> MGKRHRNLIDQITTWENLLDAYRKTSHGKRRTWGYLEFKEYDLANLLALQAELKAGNYERGPYREFLVYEPKPRLISALEFKDRLVQHALCNIVAPIFEAGLLPYTYACRPDKGTHAGVCHVQAELRRTRATHFLKSDFSKFFPSIDRAALYAMIDKKIHCAATRRLLRVVLPDEGVGIPIGSLTSQLFANVYGGAVDRLLHDELKQRHWARYMDDIVVLGDDPEELRAVFYRLRDFASERLGLKISHWQVAPVSRGINFLGYRIWPTHKLLRKSSVKRAKRKVANFIKHGEDESLQRFLASWSGHAQWADTHNLFTWMEEQYGIACH;>[5x]MEPIEEATKCYDQMLIVERYERVISYLYPIAQSIPRKHGVAREMFLKCLLGQVELFIVAGKSNQVSKL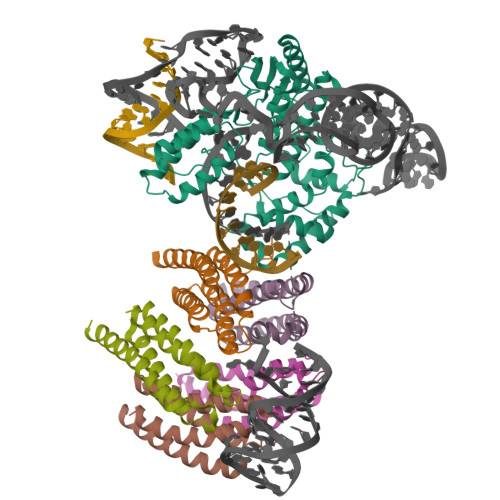YAADAGLAMLRFWLRFLAGIQKPHAMTPHQVETAQVLIAEVGRILGSWIARVNRKGTKVQVGEALVGDGNEVAHIDLIIGPRGSPAETAFCNGLVNNKHGFTSLLAVIAPNLPCKPNTLMFNKVTINDARQAVQMFGPAQHGVAMAVQDAVAEGIIPADEADDLYVLVGVFIHWEAADDAKIQKYNYEATKLSIQRAVNGEPKASVVTEQRKSATHPFAANA> DPAIVQCAW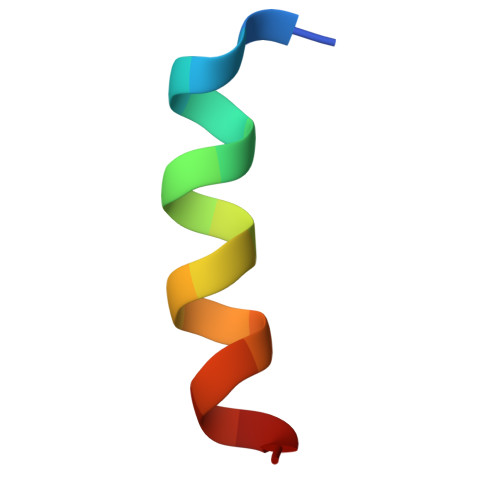AALYCDMQ>HHHHHHSSGLVPRGSHMQTTTVYSLEDLLPYLKQDNVDVKLAPGTYNVNGFDVGEDRLFSTTPLFLFEGSNSTYDFTDVKLNINTVVLTKFGNNEVNEIQILGNNNVLKNLKLEDIGTTAPSNRAQSIVIDGRDNRIEGFHLTIRGSYPYGYGDAFGKGGGSVINHRKHSGVLIRGLRNHLKDCTIISRSYGHIVFMQAASYPTVEGCYIEGEMRSTDDMLAEEGTGSPADKVDFMTVWGYKLPAGYMMSLQEGGIRAANAGTTYIDGVEIQRATDNPTVLNCTIKNARTGVTLAHANGTKYVEGCTVLGCENGYSIGSGTVVNCGADAIYGPVFKNTYGSDKGYNADITILPPSD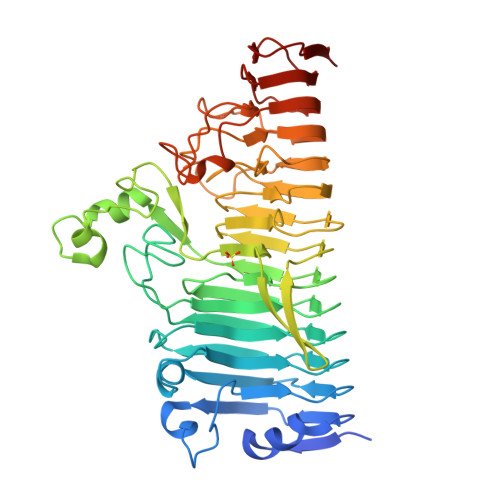AYYNGHDAVAYIGGSNHNLTFRSEITEIPSNLKIMVSGDLQGLRVLHGSNPSQNNFAGTNIVLRNLTNFPVDLHSDSSNITVTSCDTDNITDNGTNNSIEAID[2x]> GHMGAPAPVVVCYPGGAVNERDADQAMDAMLRVVERVGQWPEKSFSSVFTAKVADCGKLMAEMKPAFAITSLALYLDMRGQYDLVPVVQPRIDGRTSERYRVVAKQGRFHDMDELKGRTLGGTMLDEPAFLGKIVFAGKYDPEKDFALQPSRQAIRALRSLDKGELDAVVLNEQQFAGLSALQLASPVETVFTSAEIPLMGVVANARLTSAQERARFAQALETLCADPEGRKLCDLFGIQSFVAVDPTVFDPMARLWLARN

The aerobic methanotroph Methylococcus capsulatus was the first bacterium shown to synthesize sterols, producing a mixture of C-4 methylated sterols that are distinct from those observed in eukaryotes. C-4 methylated sterols are synthesized in the cytosol and localized to the outer membrane, suggesting that a bacterial sterol transport machinery exists. In this study, we present three putative bacterial sterol transport proteins in M. capsulatus that exhibit remarkable specificity for C-4 methylated sterols. We first used bioinformatics to identify a cytoplasmic membrane protein (BstA), periplasmic protein (BstB), and outer membrane associated protein (BstC).

BstB belongs to a family of periplasmic/substrate binding proteins (SBPs/PBPs) known to traffic bacterial metabolites such as phosphonate. The 1.6 Å-resolution structure of was determined by experimental phasing, producing electron density that allowed the unambiguous building of a model of BstB (except for one disordered loop spanning residues 202–204). The structure comprises two globular α/β domains (domains A and B) that form a cleft at the middle. The domains are connected by two loops: one 9-residue loop that runs from β4 in domain A to β5 in domain B, and a second 8-residue loop that connects β9 in domain B and β10 in domain A. These two long loops could work as a hinge to allow a bending motion of two domains to induce a conformational change upon substrate binding; this is often observed with SBPs/PBPs. The cleft between domains A and B forms a bulky cavity with an area of ~1179.5 Å2 and a volume of ~1009.6 Å3 that extends into domain A and is only accessible to solvent from one side of the structure. The cavity is predominantly hydrophobic, suggesting large and hydrophobic substrates like sterols are favorable for binding. The cleft in BstB is less open (~10 Å) than that in apo-PhnD (~22 Å). One of these patches in the central cleft could be modeled with a chloride ion engaging in polar interactions with the surrounding Glu118, Tyr120, and Phe150. In this docking model, the sterol was positioned in the hydrophobic cavity in domain A with the polar head pointing toward the central cleft and domain B, adjacent to three residues: Glu118, Tyr120, and Asn192. In contrast, the simulation (150 ns) on the MonoC docked complex which had a RMSD of 2.6 Å for the entire length of the trajectory and did not show the same conformational change as the apo-BstB simulation, which supports the idea that the apo-BstB structure represents a ‘partially-open’ form of the protein.> TPERVWNDFMTNTGNLI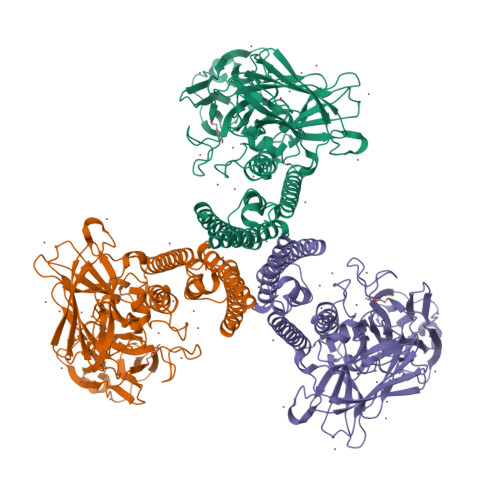DQTVTAYVRTDANAKMTVVKDYLDQYTTKFNTWKREPNNQSYRTAVITQFNLTSAKLRETAVYFSNLVGYELLLLPIYAQVANFNLLLIRDGLINAQEWSLARSAGDQLYNTMVQYTKEYIAHSITWYNKGLDVLRNKSNGQWITFNDYKREMTIQVLDILALFASYDPRRYPADKIDNTKLSKTEFTREIYTALVESPSSKSIAALEAALTRDVHLFTWLKRVDFWTNTIYQDLRFLSANKIGFSYTNSSAMQESGIYGSSGFGSNLTHQIQLNSNVYKTSITDTSSPSNRVTKMDFYKIDGTLASYNSNITPTPEGLRTTFFGFSTNENTPNQPTVNDYTHILSYIKTDVIDYNSNRVSFAWTHKIVDPNNQIYTDAITQVPAVKSNFLNATAKVIKGPGHTGGDLVALTSNGTLSGRMEIQCKTSIFNDPTRSYGLRIRYAANSPIVLNVSYVLQGVSRGTTISTESTFSRPNNIIPTDLKYEEFRYKDPFDAIVPMRLSSNQLITIAIQPLNMTSNNQVIIDRIEIIPITQSVLDET> TDKEYISEEVQKAIDDSVKQV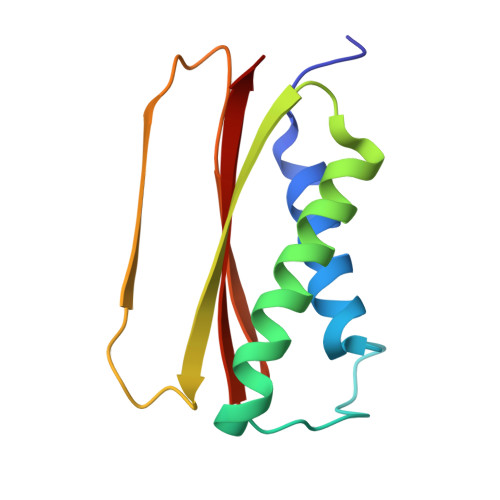FGIKDDSSQVTITYNKDKVNLWTQQIIDYTIRGLNKLGKHFKYCVTAILQQTNHAGISVQITAYQDTNTDGSLIQCYEINDIYAIVSVFAMAV Here we report a functional and structural genomics effort that applied saturation-level transposon mutagenesis and next generation sequencing (Tn-seq) to identify essential genes in B. thailandensis, followed by high-throughput structure determination. We used an “ortholog rescue” approach to maximize structural coverage of these gene families, which are likely to be essential not only in B. thailandensis, but also in related, but more virulent, Burkholderia species, such as B. pseudomallei. Using only seven Burkholderia species to select orthologs of essential genes, we solved structures for 49/406 essential gene families, and for 56 total Burkholderia protein targets (including seven ortholog replicates). Of these 56 targets, 25 satisfied criteria for being a potential antimicrobial drug target.

For the seven pairs of ortholog structures (with no bound ligand) solved in this study, the average overall Cα RMSD was 1.5±0.5 Å, indicating a high degree of structural similarity. This structural similarity suggests that the ortholog approach is an efficient method to obtain useable structures from otherwise intractable targets, thereby lowering the barrier to structure-based drug design targeting infectious organisms.

>GPGSMNVAISPGVTAGNSLPFVLFGGINVLESLDFTLDVCGEYVAVTRKLGIPFVFKASFDKANRSSIHSYRGVGLDEGLKIFAEVKARFGVPVITDVHEAEQAAPVAEIADVLQVPAFLARQTDLVVAIAKAGKPVNVKKPQFMSPTQLKHVVSKCGEVGNDRVMLCERGSSFGYDNLVVDMLGFRQMAETTGGCPVIFDVTHSLQCRDPLGDASGGRRRQVLDLARAGIAVGIAGLFLEAHPDPDRARCDGPSALPLHQLEGLLSQMKAIDDLVKRMPALEIR[4x]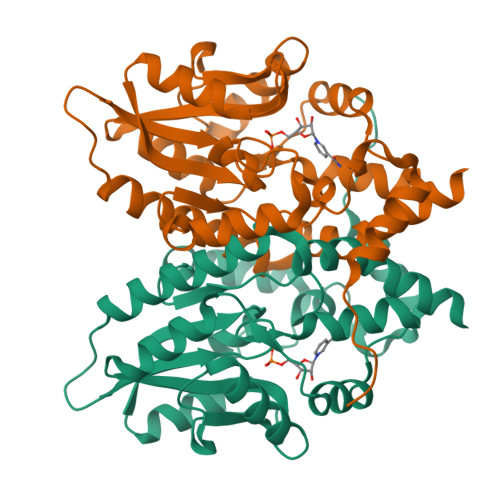> MGSHQMKSEEHANMQLQQQAVLGLNWMQDSGEYKALAYQAYNAAKVAFDHAKVAKGKKKAVVADLNETMLDNSPYAGWQVQNNKPFDGKDWTRWVDARQSRAVPGAVEFNNYVNSHNGKVFYVTNRKDSTEKSGTIDDMKRLGFNGVEESAFYLKKDKSAKAARFAEIEKQGYEIVLYVGDNLDDFGNTVYGKLNADRRAFVDQNQGKFGKTFIMLPNANYGGWEGGLAEGYFKKDTQGQIKARLDAVQAWDGKLEHHHHHH> MGEGPELHLASQFVNEACRALVFGGCVEKSSVSRNPEVPFESSAYRISA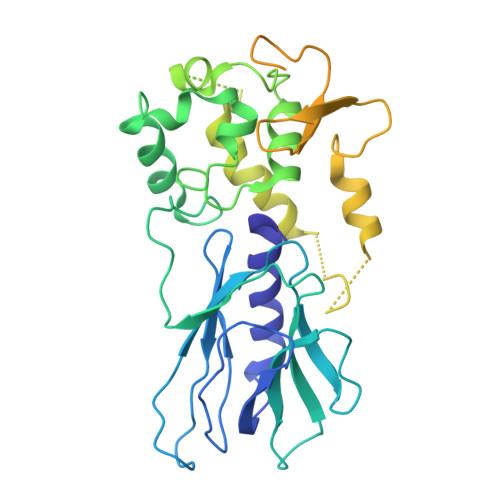SARGKELRLILSPLPGAQPQQEPLALVFRFGMSGSFQLVPREELPRHAHLRFYTAPPGPRLALCFVDIRRFGRWDLGGKWQPGRGPCVLQEYQQFRENVLRNLADKAFDRPICEALLDQRFFNGIGNYLRAEILYRLKIPPFEKARSVLEALQQHRPSPELTLSQKIRTKLQNPDLLELCHSVPKEVVQLGGRGYGSESGEEDFAAFRAWLRCYGMPGMSSLQDRHGRTIWFQGDPGPLAPKGRKSRKKKSKATQLSPEDRVEDALPPSKAPSRTRRAKRDLPKRTATQRPEGTSLQQDPEAPTVPKKGRRKGRQAASGHCRPRKVKADIPSLEPEGTSASAALGHHHHHH>[2x]FG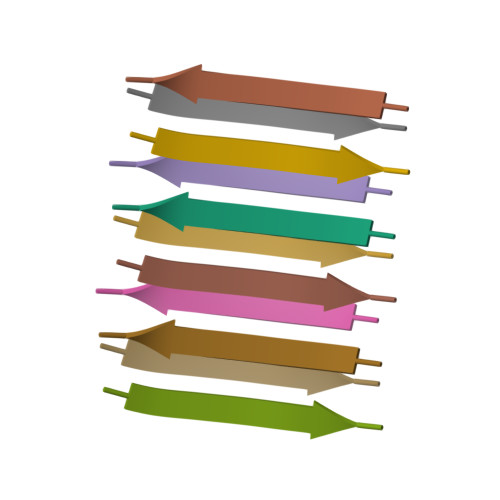AILSS> EEGLDFPEYDGVDRVINVNAKNYKNVFKKYEVLALLYHEPPEDDKASQRQFEMEELILELAAQVLEDKGVGFGLVDSEKDAAVAKKLGLTEEDSIYVFKEDEVIEYDGEFSADTLVEFLLDVLEDPVELIEGERELQAFENIEDEIKLIGYFKNKDSEHYKAFKEAAEEFHPYIPFFATFDSKVAKKLTLKLNEIDFYEAFMEEPVTIPDKPNSEEEIVNFVEEHRRSTLRK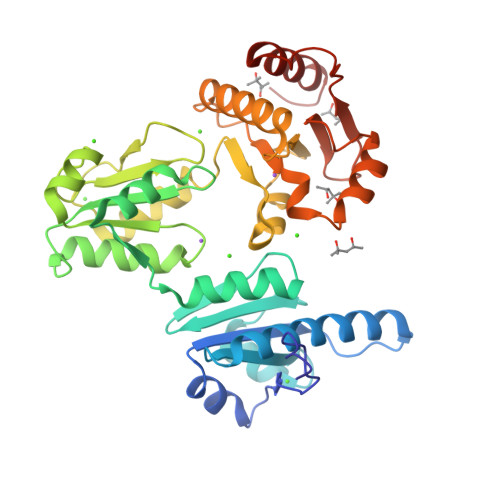LKPESMYETWEDDMDGIHIVAFAEEADPDGYEFLEILKSVAQDNTDNPDLSIIWIDPDDFPLLVPYWEKTFDIDLSAPQIGVVNVTDADSVWMEMDDEEDLPSAEELEDWLEDVLEGEINT> TQVAKKILVTCALPYANGSIHLGHMLEHIQADVWVRYQRMRGHEVNFICADDAHGTPIMLKAQQLGITPEQMIGEMSQEHQTDFAGFNISYDNYHSTHSEENRQLSELIYSRLKENGFIKNRTISQLYDPEKGMFLPDRFVKGTCPKCKSPDQYGDNCEVCGATYSPTELIEPKSVVSGATPVMRDSEHFFFDLPSFSEMLQAWTRSGALQEQVANKMQEWFESGLQQWDISRDAPYFGFEIPNAPGKYFYVWLDA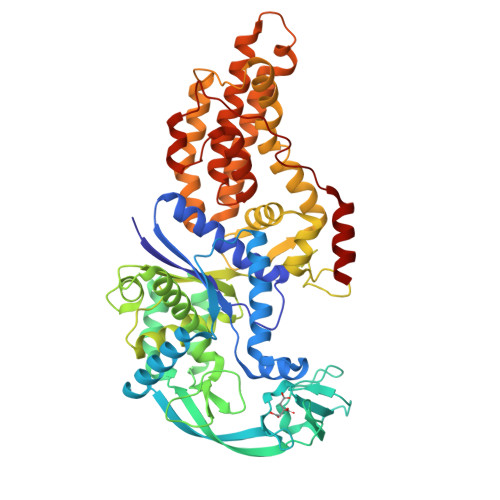PIGYMGSFKNLCDKRGDSVSFDEYWKKDSTAELYHFIGKDIVYFHSLFWPAMLEGSNFRKPSNLFVHGYVTVNGAKMSKSRGTFIKASTWLNHFDADSLRYYYTAKLSSRIDDIDLNLEDFVQRVNADIVNKVVNLASRNAGFINKRFDGVLASELADPQLYKTFTDAAEVIGEAWESREFGKAVREIMALADLANRYVDEQAPWVVAKQEGRDADLQAICSMGINLFRVLMTYLKPVLPKLTERAEAFLNTELTWDGIQQPLLGHKVNPFKALYNRIDMRQVEALVEASK> GSFDLDDVQPNKAVEPEKTKVNYTDEETQKRKKEELDKLMEPALGYVTKIPVNIPSVRKTEISEIDTVTDESLSLVPNEDKLRTIANENAGSVVTKSGSNTMNFVRSGYTIDVVHYGLRDKGYVYYKGVHPSKELPKGNIIVYQGEWDFTSNADLDAKRPNYNPEFNGYGAG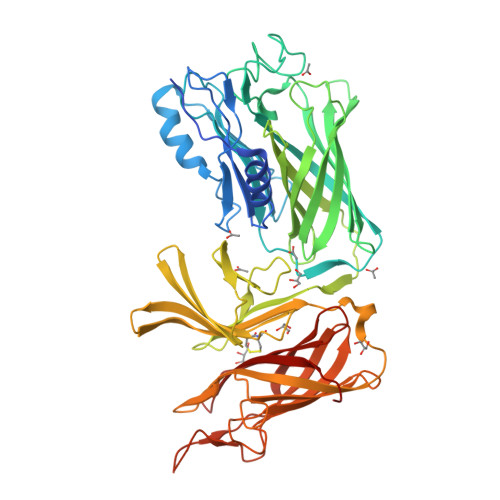QRVGVTSADAKERTYISKFNIDFSNKKLNGQLLTKTKENQEKLRYTVEANISGNRFRGKATATDKTDPILGKDSEHLEGGLYGPKSEELAGKFVAHDKSLFAVFSGKRGNDVLETVKIIDASKIDLTTFESSELNNFGNANVLIIDGQKIDLAGADFKNRKTVDINGKTMVAIACCSNLEYMKFGQLWQKEGEQTKDNSLFLQGERTATDKIPVGGNYKYVGTWDALVSKGTNWVAEADNNRESGYRSEFDVNFGDKKVSGKLFDKGGIVPVFMINADIKGNGFTGTANTTDTGFALDSGSSQHGNAVFSDIKVNGGFYGPTAGELGGQFHHKSDNGSVGAVFGAKRQIEK>NDVARGIVKADVAQNNFGLYGQGQIVAVADTGLDTGRNDSSMHEAFRGKITALYALGRTNNANDPNGHGTHVAGSVLGNATNKGMAPQANLVFQSIMDSGGGLGGLPANLQTLFSQAYSAGARIHTNSWGAPVNGAYTTDSRNVDDYVRKNDMTILFAAGNEGPGSGTISAPGTAKNAITVGATENLRPSFGSYADNINHVAQFSSRGPTRDGRIKPDVMAPGTYILSARSSLAPDSSFWANHDSKYAYMGGTSMATPIVAGNVAQLREHFVKNRGVTPKPSLLKAALIAGAADVGLGFPNGNQGWGRVTLDKSLNVAFVNETSPLSTSQKATYSFTAQAGKPLKISLVWSDAPGSTTASLTLVNDLDLVITAPNGTKYVGNDFTAPYDNNWDGRNNVENVFINAPQSGTYTVEVQAYNVPVGPQTFSLAIVH[2x];>[2x]TGAGDRHNLKTEWPELVGKSVEEAKKVILQDKP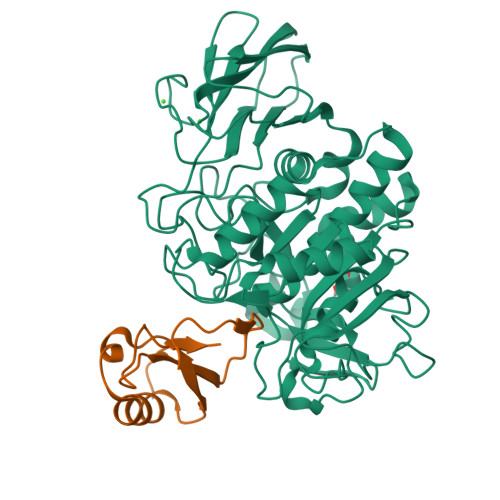EAQIIVLPVGTIVTMEYRIDRVRLFVDKLDNIAEVPRVG;> KPSLL1,3,5-BENZENETRICARBOXYLIC ACID | C9 H6 O6 | 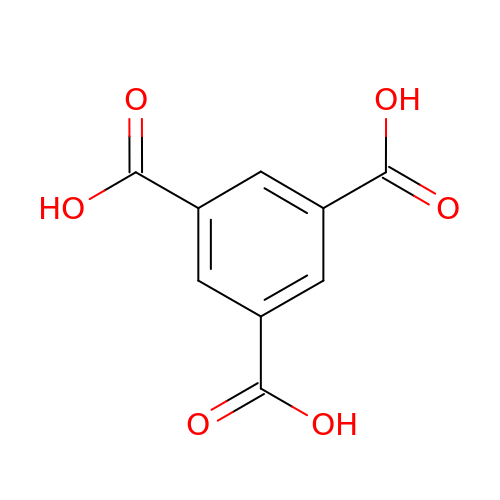QMKYBPDZANOJGF-UHFFFAOYSA-N> XD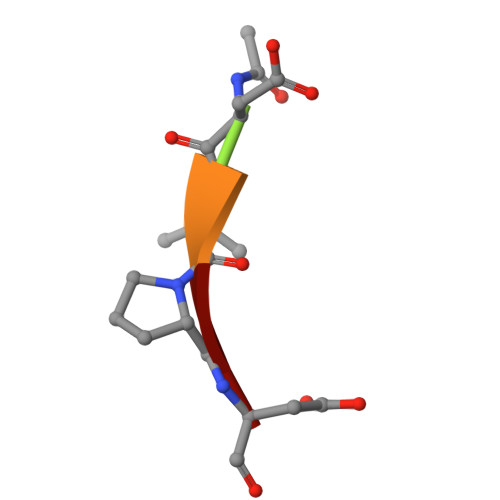VPD>[2x]GLVPRGSHMTGRMLTLDGNPAANWLNNAR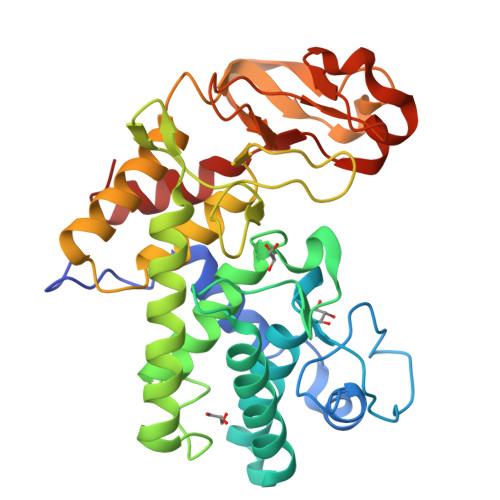TKWSASRADVVLSYQQNNGGWPKNLDYNSVGNGGGGNESGTIDNGATITEMVFLAEVYKSGGNTKYRDAVRKAANFLVNSQYSTGALPQFYPLKGGYSDHATFNDNGMAYALTVLDFAANKRAPFDTDVFSDNDRTRFKTAVTKGTDYILKAQWKQNGVLTVWCAQHGALDYQPKKARAYELESLSGSESVGVLAFLMTQPQTAEIEQAVRAGVAWFNSPRTYLEGYTYDSSLAATNPIVPRAGSKMWYRFYDLNTNRGFFSDRDGSKFYDITQMSLERRTGYSWGGNYGTSIINFAQKVGYL Guanarito virus (GTOV), first recognized in 1989, is the etiological agent of Venezuelan hemorrhagic fever. As a result of the rapid onset and high mortality rates associated with infection (∼23%), GTOV is classified as a high-priority category A biothreat agent. Together with other South American HF arenaviruses, such as Machupo virus (MACV), Junin virus (JUNV), and Sabia virus (SABV), GTOV belongs to the Tacaribe complex of the New World clade of the Arenaviridae family. The GTOV genome encodes two highly glycosylated glycoproteins which facilitate host cell attachment (GP1) and fusion (GP2). Upon acidification during clatherin-mediated endocytosis, GP1 is released from the virion and GP2 mediates fusion of the viral and host membranes.

We present here the first structure of a New World arenavirus fusion glycoprotein and show that GTOV GP2 adopts an archetypal class I-type postfusion fold. Approximately 50 residues at the N terminus of the GTOV GP2 ectodomain were removed to exclude the aggregation-inducing N-terminal hydrophobic fusion loop. To aid crystallogenesis, recombinant glycoprotein expression was performed in GlcNAc transferase I-deficient human embryonic kidney 293S (HEK 293S) cells, which traps glycosylation predominantly to a homogenous Man5GlcNAc2 glycoform. Each of the three GP2 subunits in the asymmetric unit consists of three regions: a 45-amino-acid N-terminal α-helix (residues 301 to 346), a 50-amino-acid “T region” (residues 347 to 398; named in comparison with the Old World LCMV GP2 structure), and a short C-terminal α-helix (residues 399 to 408). The N-terminal α-helix spans the entire length of the 85-Å-long molecule and connects to the C-terminal helix through the T region, which is composed of loops and a small α-helix (residues 358 to 364). The N- and C-terminal helices pack closely in an antiparallel arrangement, where each protomer associates to form a trimeric coiled coil. Our structure is in a postfusion conformation, with the N terminus (fusion loop region) and C terminus (transmembrane region) colocalized, consistent with the merger of the virion and host cell membranes. The crystal contained protein-glycan and glycan-glycan lattice contacts, which facilitated visualization of carbohydrate chains from three out of the five N-linked glycosylation sites on GP2. The T region also contains a 10-amino-acid stretch (residues 365 to 375) which is fully ordered in one protomer and disordered in the second and third. However, superposition of equivalent GTOV and LCMV protomers leads to a greater structural variation between the two structures (a 2.2-Å root mean square deviation [RMSD] over 96 Cα residues) than expected between two structures with 50% sequence identity (an ∼1.0-Å RMSD).

>TGDSEFCDMLRLFDFNKNAIEKLNNQTKTAVNMLTHSINSLISDNLLMRNKLKEVLKVPYCNYTRFWYINHTKSGEHSLPRCWLVSNGSYLNESDFRNEWILESDHLIAEMLSKEYQDRQGKTPLTLVDGTKHHHHHH[3x]Phycobilisomes (PBS) are antenna megacomplexes that transfer energy to photosystems II and I in thylakoids. Here we show the cryo-EM structure at a global resolution of 2.9 Å of the 5.9-MDa PBS from Anthocerotibacter panamensis (hereafter A. panamensis), a recently discovered Gloeobacterial species that diverged from Gloeobacter spp. around 1.4 billion years ago. The A. panamensis PBS features a configuration comprising two herein characterized linkers and presents a paddle-shaped morphology. The two-fold symmetric PBS contains twelve APC hexamers assembled as a heptacylindrical core surrounded by twelve PC hexamers, with approximate dimensions of 273 Å (width), 500 Å (height), and 129 Å (thickness).

The cryo-EM map illustrates that the heptacylindrical core comprises a pentacylindrical core (A, A’, B, B’, C, and C’) with two additional core cylinders (D and D’) on the top. The two top core cylinders are assembled with ApcA1, ApcA2, ApcB1, ApcB2, and ApcC1, in which (ApcA1/ApcB1)3 form all trimers except that D3 and D'3 are formed by (ApcA2/ApcB2)3. Interestingly, ApcA1 is not in the same clade with other ApcA and ApcD subunits, and ApcB1 is not in the same clade with other ApcB and ApcF subunits. The lack of orthologs of ApcA1 and ApcB1 in crown Cyanobacteria suggests that the top two core cylinders were lost during the evolution to crown Cyanobacteria. A core-core linker, ApcH (LCC), connects the top and bottom cylinder complexes. However, unlike ApcE, ApcH does not have the pfam00502 domain that binds PCB and anchors the PBS to the thylakoid membrane. Instead, the N-termini of the two ApcH copies attach to the C and C’ of the pentacylindrical core, leading to the giant heptacylindrical core and expanding the overall light-harvesting cross section. Overall, the top two core cylinders add 48 additional PCB chromophores to the core, thereby expanding the absorption cross-section for red light. The top core cylinders (D/D’) are essential to connect the energy transfer from the chains and the top side PC hexamers to the pentacylindrical core. The assembly of ApcA2 and ApcB2 in the D'3 position is essential for the function of the PBS because the D'3 trimer mediates energy transfer from the chain to the core.

>[2x]MQPIILRTLSARRPVQGRPNLETYTSEVERWKAIAQTQYALELAKEMSRPALRTSVGDLPGGLWGVRPGFQSPPKQRYRWTLKQSKAEKEALLEAIYRQVLERVLPEGSRLNEEESRLNNGDITVREFVRRLASSDLYVQSFLVRYPNTKLVEKLYKHLLGRAPSNQKEIIKYHDLLARKGLKAAVDAMVTTEEYTEIFGDDTVPFARYTTDPAHGLVTQAYLGGVLVNAKHTYQNRTLNFPSYGPGSQTGGEQRSLPLVPERVFSLGDGASVDQILRASYRQILEKEPQELQRLSVAESQLRNGEISVKEFIRALGYSEIYAKFFLARWYNGKVAEFNFKHFLGRQPASATELGSHITLIGTKGLKVAIDTLLASQEYQDNFGDDTVPYYRLQAERYVGTTDAPSRAYVLARSRVQTALNKPTVPSYSLV;>MSAITKAILNADAEARYLSPGEIDVVRGYLASGERRVRVARVLSDNALRIVRGAGDTMFQKRPDLVAPGGNAYGEVRTAKCLRDLDYFLRLVTYGVLAGDTSPIDEIGLIGIKETYSLLEVPVPGVIDGIKAAKQQAAALLSSEDAAEASFYFDYVISAMS[18x];>[6x]MSVVTKAIVSADAEARYLSPGELDRIRGFVSSGERRLRVAQTLTESRERIIKQAGDQLFQKRPDLVSPGGNAYGAERTASCLRDLDYYLRLVTFGIVAGDVTPIEEIGVIGVKEMYRNLEVPLPGMVEAVKAMKSVATGLLSGDDSAEVGYYFDYLAGALA;>MLDAVTKIINRTDAEGRYFASKDFDEVTRFFATGEARLRAASTISANAASILRESAAALFTEQPDLLRPGGNAYTSRRYAACVRDMEYFLRYATYALVAGDTSVIDERVLNGLKETYMSLGVPIPSTVAGVTAMKGVVASMIGSEANVYFDHIAKGLS[18x];>MQDAITSVINTYDVQGKYFDTSAFDKLKAYYATGELRVRAAGTISANAATIIKEASAKLFSNQPDLVRPGGNAYTTRRYAACVRDMDYFLRYATYAMLAGDTSILDERVLNGLKETYNSLGVPISSTVQGIQAMKEVTGSLVGSGAAKEMGVYFDYLSSGLS[6x];>MARTISITACVPRRTKSVGASREIQNVYFTKRISFDQFTPEYQRIHRQGGTILNVQCMGS[4x]>VDSVYRTRSLGVAAEGIPDQYADGEAARVWQLYIGDTRSRTAEYKAWLLGLLRQHGCHRVLDVACGTGVDS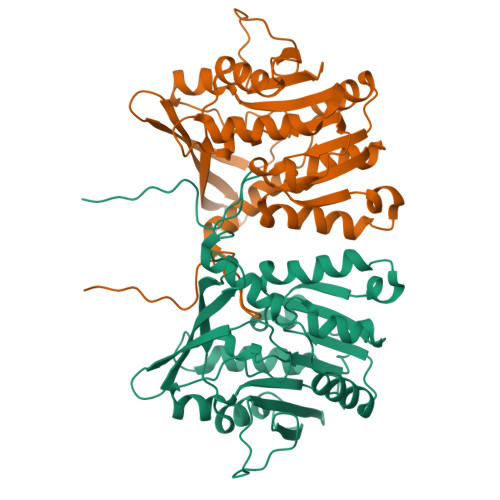IMLVEEGFSVTSVDASDKMLKYALKERWNRRKEPAFDKWVIEEANWLTLDKDVPAGDGFDAVICLGNSFAHLPDSKGDQSEHRLALKNIASMVRPGGLLVIDHRNYDYILSTGCAPPGKNIYYKSDLTKDITTSVLTVNNKAHMVTLDYTVQVPGAGRDGAPGFSKFRLSYYPHCLASFTELVQEAFGGRCQHSVLGDFKPYRPGQAYVPCYFIHVLKKTG[2x]>MRCIGMSNRDFVEGVSGGSWVDIVLEHGSCVTTMAKNKPTLDFELIKTEAKQPATLRKYCIEAKLTNTTTESRCPTQGEPSLNEEQDKRFVCKHSMVDRGWGNGCGLFGKGGIVTCAMFRCKKNMEGKVVQPENLEYTIVITPHSGEEHAVGNDTGKHGKEIKITPQSSITEAELTGYGTVTMECSPRTGLDFNEMVLLQMENKAWLVHRQWFLDLPLPWLPGADTQGSNWIQKETLVTFKNPHAKKQDVVVLGSQEGAMHTALTGATEIQMSSGNLLFTGHLKCRLRMDKLQLKGMSYSMCTGKFKVVKEIAETQHGTIVIRVQYEGDGSPCKIPFEIMDLEKRHVLGRLITVNPIVTEKDSPVNIEAEPPFGDSYIIIGVEPGQLKLNWFKKGSSIGQMFETTMRGAKRMAILGDTAWDFGSLGGVFTSIGKALHQVFGAIYGAAFSGVSWTMKILIGVIITWIGMNSRSTSLSVTLVLVGIVTLYLGVMVQA[3x];>SVALVPHVGMGLETRTETWMSSEGAWKHVQRIETWILRHPGFTMMAAILAYTIGTTHFQRALIFILLTAVTPSMT[3x]

The surface of mature, infectious flaviviruses is composed of an icosahedral shell of 90 flat-lying envelope (E) protein dimers, the main target of humoral immunity. In contrast to their mature counterparts, immature virions possess 60 protruding spike-like trimers of precursor membrane (prM)-E complexes (prM3E3). The pr domain of prM binds to E, obscuring the fusion peptide and thereby preventing unproductive fusion within the already infected cell. When immature virions reach the low-pH environment of the trans-Golgi network (TGN), the trimeric prM3E3 spikes rearrange into the flat-lying conformation, characteristic of the mature virus.

Considering the conservation, we wanted to assess if a lipid is present in related pathogenic flaviviruses, such as ZIKV or DENV. Because the available 3.6 Å resolution map did not resolve unambiguously the presence of a lipid, we carried out our own cryo-EM reconstruction of DENV2. The reconstruction reached a resolution of 3.1 Å and again revealed a lipid in the same region, suggesting that the binding pocket is conserved in flaviviruses. We chose to carry out mutagenesis in DENV2, as this is the more amenable system and impactful pathogen. We found that no virus could be recovered after exchange of His437 (equivalent to His447 in SPOV) to either a negatively charged glutamate or a small and neutral alanine. Similarly, we observed no virus recovery upon introducing a bulky Tyr sidechain at position Gly441 (Gly451 in SPOV). This glycine is in close contact with the lipid and any other amino-acid besides Gly would sterically displace the lipid, which may explain why it is strictly conserved at this position. Although we cannot exclude with absolute certainty that these mutations interfere with the folding of E, the results suggest that an intact lipid-binding pocket is important in the virus lifecycle, with a specific role for the adjacent histidine. Furthermore, a highly conserved and mutation-sensitive histidine (His447 in SPOV, His437 in DENV2) is located adjacent to the lipid, suggesting a pH-dependent role during the viral lifecycle.>[4x]NLPPEKKWLGTPIEEMRKMPRCGIHLPSLRPSASHTVTVRVDLLRAGEVPKPFPTHYKDLWDNKHVKMPCSEQNLYPVEDENGERTAGSRWELIQTALLNKFTRPQNLKDAILKYNVAYSKKWDFTALVDFWDKVLEEAEAQHLYQSILPDMVKIALCLPNICTQPIPLLKQKMNHSVTMSQEQIASLLANAFFCTFPRRNAKMKSEYSSYPDINFNRLFEGRSSRKPEKLKTLFCYFRRVTEKKPTGLVTFTRQSLEDFPEWERCEKPLTRLHVTYEGTIEGNGRGMLQVDFANRFVGGGVTGAGLVQEEIRFLINPELIVSRLFTEVLDHNECLIITGTEQYSEYTGYAETYRWARSHEDGSEKDDWQRRCTEIVAIDALHFRRYLDQFVPEKVRRELNKAYCGFLRPGVPSENLSAVATGNWGCGAFGGDARLKALIQILAAAAAERDVVYFTFGDSELMRDIYSMHTFLTERKLDVGKVYKLLLRYYNEECRNCSTPGPDIKLYPFIYHAVESSAET

Reversal of PARylation is predominantly carried out by poly(ADP-ribose) glycohydrolase (PARG) in nucleus and cytosol, whereas ADP-ribosylhydrolase 3 (ARH3) may play a role in mitochondrial PAR degradation. PARG comprises an N-terminal regulatory/targeting domain and a C-terminal catalytic domain. The mouse PARG catalytic domain has a bean-shaped structure, with the active site in a deep cleft in the middle on the abdominal side.

We purified and crystallized the recombinant mouse PARG catalytic domain (residues 439–959) and determined the unliganded structure of mPARG(439–959) using Se-Met SAD method at 2.0 Å resolution. A nine-strand mixed β sheet is sandwiched by two helical domains. The N-terminal helical domain has nine α helices, whereas the C-terminal helical domain has five. The core structure of the mPARG catalytic domain also has an ADPr-binding macrodomain fold, despite missing the first β strand of the macrodomain. Tyr788, a residue previously identified to be important for the recognition of the PARG inhibitor ADP-HPD, is located at the tip residue in this β hairpin pointing into the cleft. The very N-terminal segment of the mPARG catalytic domain contains the sixteen-residue putative mitochondrial targeting sequence (MTS, residues 454–469, MRKMPRCGIHLPSLRP) and binds to a groove on the side opposite to the active site. In our mPARG structures, this MTS together with residues preceding it, has an extended conformation and wraps along the back side of the PARG catalytic domain. The MTS docks in a hydrophobic groove on the back side of the β sheet, which is the opposite side from the active site. Hydrophobic residues Met454, Met457, Leu464 and Leu467 on the MTS pack tightly with this hydrophobic groove. With the first crystal form that we solved mPARG structure (space P1), both methods failed, since the active site cleft is close to another copy of the mPARG molecule in the crystal lattice.>VGYGDITQVETSGASSKTSRQDKLEYDGVR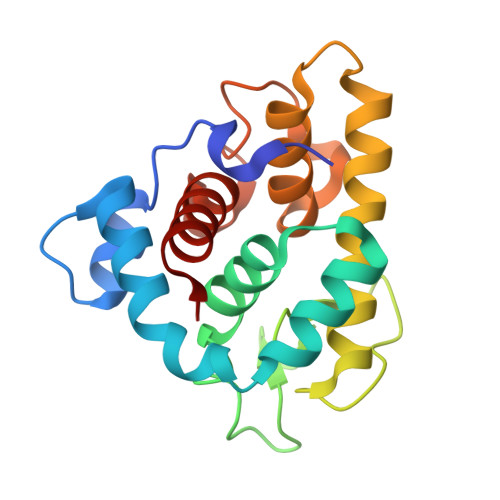ASHTMAQTDAGRMEKYKSFINNVAKKHVVDPAVIAAIISRESRAGNVIFNTTPPGWGDNYNGFGLMQVDKRYHEPRGAWNSEEHIDQATGILVNFIQLIQKKFPSWSTEQQLKGAIAAYNTGDGRVESYESVDSRTTGKDYSNDVVARAQWYKKNGF[4x]>MKFKHQGLVADLLPNIRVMQGVGHFMFNYYSEGKKFPHRIYCIVTLLLLLLQYGMMAVNLMMESDDVDDLTANTITMLFFLHPIVKMIYFPVRSKIFYKTLAIWNNPNSHPLFAESNARFHALAITKMRRLLFCVAGATIFSVISWTGITFIEDSVKRITDPETNETTIIPIPRLMIRTFYPFNAMSGAGHVFALIYQFYYLVISMAVSNSLDVLFCSWLLFACEQLQHLKAIMKPLMELSATLDTVVPNSGELFKAGSADHLRESQGVQPSGNGDNVLDVDLRGIYSNRQDFTATFRPTAGTTFNGGVGPNGLTKKQEMLVRSAIKYWVERHKHVVRLVTAVGDAYGVALLLHMLTTTITLTLLAYQATKVNGVNVYAATVIGYLLYTLGQVFLFCIFGNRLIEESSSVMEAAYSCHWYDGSEEAKTFVQIVCQQCQKAMSISGAKFFTVSLDLFASVLGAVVTYFMVLVQLK[3x];> MARLVLHEVRYVLMAMLYISRGMAKQIQNSTIDLYVYWFLTFIPIASLCVPQFTYLVVDTKSLIDFISVLVPITEILLTNGKMIICNVKRGKIINLINQVQVAWDECAKSEHLEIQTLITATAKKTKIFVIIYTTSFLLICVEYSSMPLFKLIYHSAVYGKQSNYTIALPYLSRFAYSTESTTSFAWTYFFILLGVYLLALTLSGFDSLFATLVMHVKMMFKVLKFEIEQLGLDLSAGKSHVELQAKLKQIILKHKTNLSLIEQLEDGFSFFLMAQFLTSSILVCVVLYELTMVFGWNEDTFKTVTYLPGAILQLFLFCWYAQQITEEARLVSDHIYNIPWYLADPKLQKDILTFMVKAQKPTGVTASKFYMVTLQTFQRISSTSYSYFTLLQTINQQ

Most insects, including human-targeting mosquitoes, detect odors through odorant-activated ion channel complexes consisting of a divergent odorant-binding subunit (OR) and a conserved co-receptor subunit (Orco). As a basis for understanding how odorants activate these heteromeric receptors, we report here cryo-EM structures of two different heteromeric odorant receptor complexes containing ORs from disease-vector mosquitos Aedes aegypti or Anopheles gambiae. We determined the structure of a heteromeric complex formed by ORs from these species in complex with a Apocrypta bakeri fig wasp Orco that is amenable to structural determination. We find that these complexes form asymmetric tetramers containing 1 OR and 3 Orco subunits, where activation of the sole OR subunit upon ligand binding suffices to open the ion conduction pathway.

To determine if the 1:3 subunit stoichiometry can be observed with other members of the OR family, we turned to studying the OR28 receptor of An. gambiae, a main vector of malaria, that responds to the natural odorants acetophenone (a plant volatile) and 2,4,5-trimethylthiazole (henceforth TMT; an animal odor, originally isolated from anal secretions of mammals). The cryo-EM dataset of the unbound structure also contains an active state, suggesting that, like the AaOR10/Orco complex, the AgOR28/Orco complex exists in an equilibrium between states in the absence of odorant. Overall, subunit stoichiometry, mechanism of pore opening and ligand binding of the AgOR28/Orco complex largely resembles the observations of the AaOR10/Orco complex, suggesting that these might be conserved features of this family of proteins.> MATAQLQRTPMSALVFPNKISTEHQSLVLVKRLLAVSVSCITYLRGIFPECAYGTRYLDDLCVKILREDKNCPGSTQLVKWMLGCYDALQKKYLRMVVLAVYTNPEDPQTISECYQFKFKYTNNGPLMDFISKNQSNESSMLSTDTKKASILLIRKIYILMQNLGPLPNDVCLTMKLFYYDEVTPPDYQPPGFKDGDCEGVIFEGEPMYLNVGEVSTPFHIFKVKVTTERERMENIDSTILSPKQIKTPFQKILRDKDVEDEQEHYTSDDLDIETKMEEQEKNPASSELEEPSLVCEEDEIMRSKESPDLSIS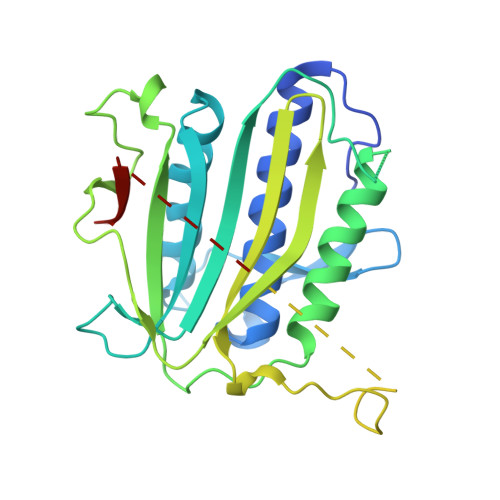HSQVEQLVNKTSELDMSESKTRSGKVFQNKMANGNQPVKSSKENRKRSQHESGRIVLHHFDSSSQESVPKRRKFSEPKEHI> RMNELKHAVVPIDLQSFCLEGTLALW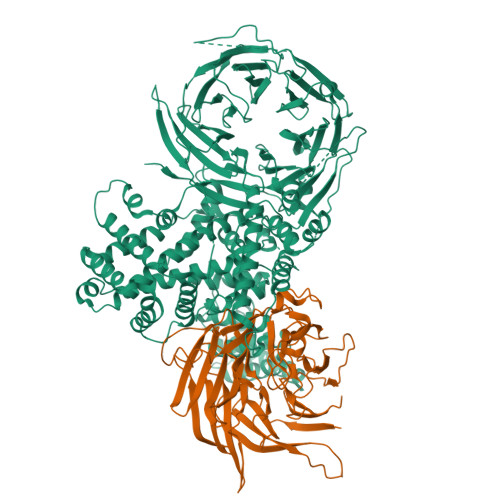VPALENDSEDDSEAIETADDNEKLFKKECVAYDAGVYTSNKSKGSQTLRWSIFQNRTLTIFDVSLNSKKEPLSKFNVKIHFPSNVMKDGVAFSFSEHSDTTIIYAITHARVLYYIRLSKTWFQLPDARLDDDWCLCYRPISFLNQKPDLMAAISTSEICVSFFNGGLTKIILNPKDASHYEQHIDDSSYLFSLKKYLSLQAFKADYRSPNTIISMIFLSTYNVLVMLSLDYKLKVLDLSTNQCVETIELSQTILPLQSFPYLTSDHTTNSFIALYYPDNSHGSFSIYKLNANAHSFKLNVVIEKGIIPPSLPDDEFIPWMLSDFQLISSEGSQSKFLLIIAWKSNLNTVIQKCNLSLDQDESFSCVWSHSLDSFSLIEKTFFDVPTNMSSGDISEIWLQHIFAHNTSIESIQVALLSFQNSSSQVSKNKLDKFGALTISELKNAVLSSIVSTIQIEPNSDLTGYDYYEYKRLLYNEWERFAKLVAYLDHFGDEILSINFDPSNAVTYINYANKVAFIRDPYLIESFDEEPLTKLISSLETDDPSLIEGYQILDLGRSLHSCMSFSTLSEIRYSLRELVQDLPSYSLFDTLWVFYDKHIYPNVDPDYISTLIDTLVSLENPMRDIDSLIQRLRSFDIYNHSAQSPSLFLCASVARVLDSILKKFQVSIEGFIFLLSLITSQQDYELQSKFAGCDKLFLSLLEDWRLVSFLLENSALLLEKFEEEDVDSTNCNLNTMEALASVNTALQFFSALNYSECFSESQISPLHATVISSLSAIFIRDDTENDLVTELVEKLFLFKQYNACMQLIGWLNSDPIAVYLKALIYLKSKEAVKAVRCFKTTSLVLYSHTSQFAVLREFQEIAEKYHHQNLLSCYYLHLSKKLFEESAYIDALEFSLLADASKETDDEDLSIAITHETLKTACAAG;> GSMTLSSNQYQLPLNVRPYTTTWCSQSPSCSNLLAIGHDTGITIYCASEEQTPGSTGLTLQELFTIQTGLPTLHLSFSSSCSYSENLHDGDGNVNSSPVYSLFLACVCQDNTVRLIITKNETIITQHVLGGKSGHHNFVNDIDIADVYSADNRLAEQVIASVGDDCTLIIWRLTDEGPILAGYPLSSPGISVQFRPSNPNQLIVGERNGNIRIFDWTLNLSAEENSQTELVKNPWLLTLNTLPLVNTCHSSGIASSLANVRWIGSDGSGILAMCKSGAWLRWNLFANNDYNEISDSTMKLGPKNLLPNVQGISLFPSLLGACPHPRYMDYFATAHSQHGLIQLINTYEKDSNSIPIQLGMPIVDFCWHQDGSHLAIATEGSVLLTRLMGFTRL>[8x]SNAMKKAKSRIAILGTGGTIAGFIDSTIATTGYAAGAIDIDVLIKAVPQIRDLADISWEQIANIDSSNMCDEIWLRLAKKIAKLFAEGIDGVVITHGTDTMEETAYFLNLTIKSDKPVVLVGAMRPSTAISADGPKNLYNAVALV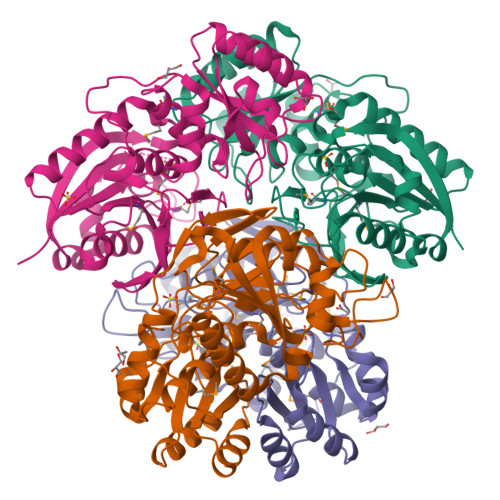VNKEAKNKGVMVAINDKILSARGVVKTHSLNVDAFSSPDFGDLGYIVDGKVFFYNNVIKAHTKNAPFDVSKLTSLPKVDILYSYSNDGSGVAAKALFEHGTKGIVVAGSGAGSIHKNQKDVLKELLKKGLKVVVSSRVVAGCVAVSDSDEKLGFISAEDLNPQKARVLLMLALTKTSDPKKIQEYFLKY>GMTRPAHPISRYPVPELAALPDDIRQRILEVQDKAGFVPNVFLTLAHRPDEFRAFFAYHDALMLKDGGLTKGEREMIVVATSAANQCLYCVVAHGAILRIYEK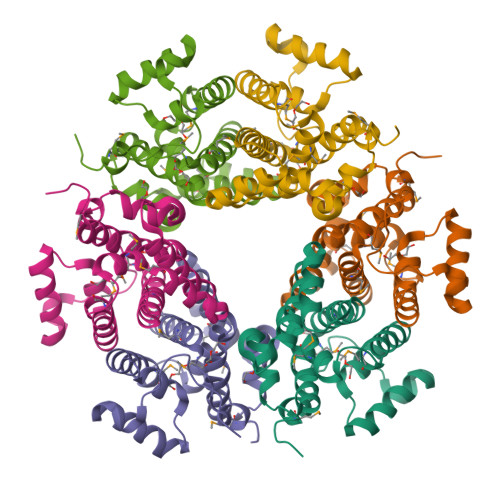KPLVADQVAVNYLKADIPPRQRAMLDFALKVCKASHEVNEADFEALREHGFTDEDAWDIAAITAFFGLSNRMANTIGMRPNDEFFLMGRVPKSK[12x]> GAMAVNAVHLESDAFLVCMNHALSTEKEEVMGLCIGEVDTNRIVHIHSVIILRRSDKRKDRVEISPEQLSAASTEAERLAEMTGRPMRVVGWYHSHPHITVWPSHVDVRTQAMYQMMDQGFVGLIFSCFIEDKNTKTGRVLYTCFQSVQAQKGSEYERIEIPIHVVPHEAIGKVCLESAVELPRILCQEEQDTYRRIHSLTHLDPITKIHNGSVFTKNLCSQMSAIS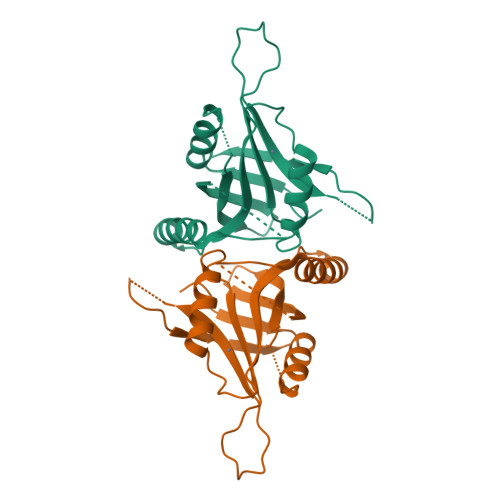GPLLQWLEDRLEQNKQSIITLQKEKELLTQELAAL> ERFAREPMAAGHRMWQMAGLKAQRAQTDVNNKKAAFDAAAKEKSDADVALSSALERRKQKENKEKDAKAKLDKESKRNKPGKATGKGKPVNNKWLNNAGKDLGSPVPDRIANKLRDKEFKSFDDFRKKFWEEVSKDPELSKQFSRNNNDRMKVGKAPKTRTQDVSGKRTSFELHHEKPISQN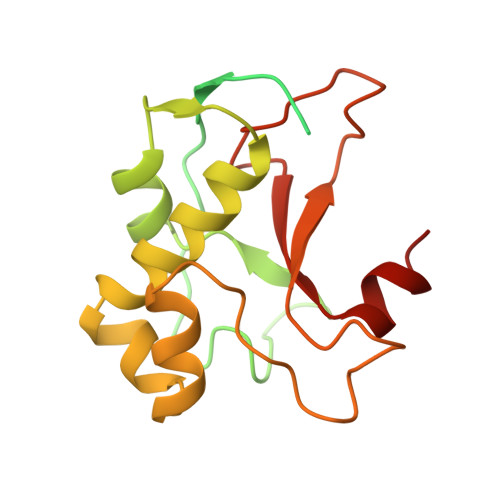GGVYDMDNISVVTPKRHIDIHRGK>MAHHHHHHMSTTVIILAAGKGTRMRSQLPKVLQPLAGRPLLGHVIKTAKQLLAENIITIYGHGGDHVKKTFAQENIQWVEQAEQLGTGHAVQMTLPVLPKDGISLILYGDVPLVRQTTLEQLIEVSNKTGIGMITLHVDNPTGYGRIVRQDGKIQAIVEHKDATEAQRQIQEINTGIYCVSNAKLHEWLPKLSNENAQGEYYLTDIVAMAVADGLEIASIQPELAFEVEGVNDRLQLAALEREFQKQQAKELMQQGVTFADPARFDLRGTVKVGHDVRIDVNVIIEGNC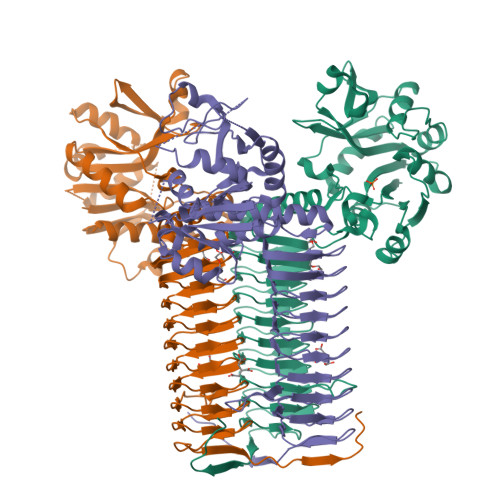ELGDFVEIGAGCILKNTTIAAGTKVQAYSVFDGAVVGENTQIGPFARLRPGAKLANEVHIGNFVEVKNTTIGLGSKANHFTYLGDAEIGAESNIGAGTITCNYDGANKHKTTIGDAVFIGSNSSLVAPVTIGNGATVGAGSVITKDVAEQSLSFERAQQISKANYQRPQKLKK[3x]> MILFDKNKRILKKYAKMVSKINQIESDLRSKKNSELIRLSMVLKEKVNSFEDADEHLFEAFALVREAARRTLGMRPFDVQVMGGIALHEGKVAEMKTGEGKTLAATMPIYLNALIGKGVHLVTVNDYLARRDALWMGPVYLFLGLRVGVINSLGKSYEVVWKNPDLARKAIEENWSVWPDGFNGEVLKEESMNKEAVEAFQVELKEITRKEAYLCDVTYGTNNEFGFDYLRDNLVLDYNDKVQRGHFYAIVDEADSVLIDEARTPLIISGPSKESPSVYRRFAQIAKKFVKDKDFTVDEKARTIILTEEGVAKAEKIIGVENLYDPGNVSLLYHLINALKALHLFKKDVDYVVMNGEVIIVDEFTGRLLPGRRYSGGLHQAIEAKEGVPIKEESITYATITFQNYFRMYEKLAGMTGTAKTEESEFVQVYGMEVVVIPTHKPMIRKDHDDLVFRTQKEKYEKIVEEIEKRYKKGQPVLVGTTSIEKSELLSSMLKKKGIPHQVLNAKYHEKEAEIVAKAGQKGMVTIATNMAGRGTDIKLGPGVAEL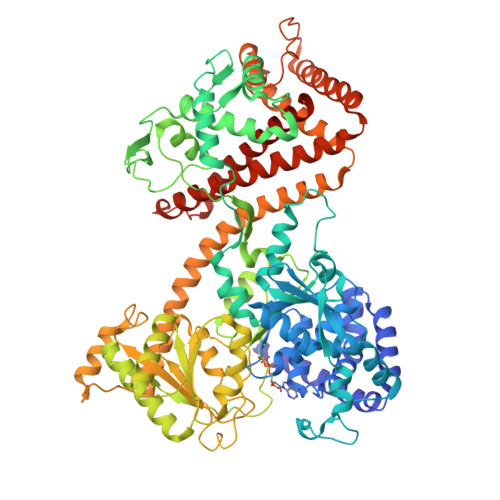GGLCIIGTERHESRRIDNQLRGRAGRQGDPGESIFFLSLEDDLLRIFGSEQIGKVMNILKIEEGQPIQHPMLSKLIENIQKKVEGINFSIRKTLMEMDDVLDKQRRAVYSLRDQILLEKDYDEYLKDIFEDVVSTRVEEFCSGKNWDIESLKNSLSFFPAGLFDLDEKQFSSSEELHDYLFNRLWEEYQRKKQEIGEDYRKVIRFLMLRIIDDHWRRYLEEVEHVKEAVQLRSYGQKDPIVEFKKETYYMFDEMMRRINDTIANYVLRVHHHHHH>[3x]MVNTVNYFKQKLKTEQQIGMWVGLADGYCAEIAANVGYDWLLIDGEHAPNDVRSILAQLQSIAAYPSQAVVRPVSGDVPLIKQLLDIGAQTLLIPMVESAEQAELMVKATRYPPEGIRGVGAALARASRWNNISDYLQTADEQICLLVQVESKKGLDNLDEILNVDGVDGIFIGPADLSAALGYRGNPGHEFVQNIIVQTIQKIRAAGKAAGILSADEKLAKQYLELGTEFVAVGVDTSLLMKSMKQLLSKFKNVDGPVSTSPSVY

Here, we investigated a new Class II metal aldolase from the p-hydroxyphenylacetate degradation pathway in Acinetobacter baumannii, 4-hydroxy-2-keto-heptane-1,7-dioate aldolase (AbHpaI), which has various properties suitable for biocatalysis, including stereoselectivity/stereospecificity, broad aldehyde utilization, thermostability, and solvent tolerance. For Class II metal aldolases, the enzyme uses a divalent metal ion (M2+) as a cofactor for substrate binding and stabilization of an enolate intermediate, which allows the reaction to proceed through C-C bond formation or cleavage. Each protomer contains eight β/α motifs of a TIM barrel fold with an additional α-helix (residues 6–11; N-helix) at the N-terminus. Three protomers are associated in a tight trimeric structure to generate three catalytic pockets, and the trimer is dimerized to form a stable and rigid hexamer with 35% buried area.

Ca2+ ion was found abundantly in purified AbHpaI. However, it does not act as a cofactor to enhance enzyme catalysis. Therefore, the function of Ca2+ ion in AbHpaI was further investigated by analyzing the enzyme structure in complex with Ca2+. Therefore, Ca2+ functions to prevent repulsive forces and to reduce movement of the (β/α)2 loop in AbHpaI where Asp51 sits. Consequently, by stabilizing the (β/α)2 loop where the active residues Glu46 and His47 reside (see proposed mechanisms), Ca2+ could indirectly aid in the catalysis of AbHpaI. Apart from the catalytic Zn2+, our structural data demonstrates that Ca2+ is found at the trimer center on the dimerization interface of the AbHpaI hexamer, neutralizing the negative charges of three Asp51 carboxylate side chains, which is unique for AbHpaI and is not found in EcHpaI, SwHpaI, other pyruvate-specific Class II metal aldolases. The results showed that apo-AbHpaI is quite thermostable naturally with a protein melting temperature (Tm) value as high as 81.3 °C. The binding of transition M2+, but not alkaline earth M2+, can further increase the thermostability of apo-AbHpaI.6-chloro-1,3-dihydro-2H-indol-2-one | C8 H6 Cl N O | 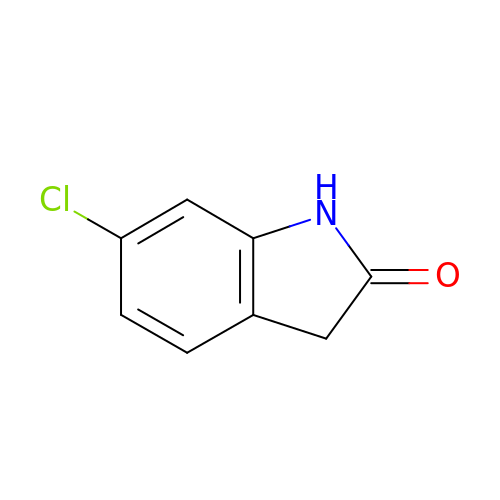CENVPIZOTHULGJ-UHFFFAOYSA-N> SEQHAQGADAVVDLNNELKTRREKLANLREQGIAFPNDFRRDHTSDQLHAEFDGKENEELEALNIEVAVAGRMMTRRIMGKASFVTLQDVGGRIQLYVARDDLPEGVYNEQFKKWDLGDILGAKGKLFKTKTGELSIHCTELRLLTKALRPLPDKFHGLQDQEARYRQRYLDLISNDESRNTFKVRSQILSGIRQFMVNRGFMEVETPMMQVIPGGAAARPFITHHNALDLDMYLRIAPELYLKRLVVGGFERVFEINRNFRNEGISVRHNPEFTMMELYMAYADYKDLIELTESLFRTLAQDILGKTEVTYGDVTLDFGKPFEKLTMREAIKKYRPETDMADLDNFDSAKAIAESIGIHVEKSWGLGRIVTEIFEEVAEAHLIQPTFITEYPAEVSPLARR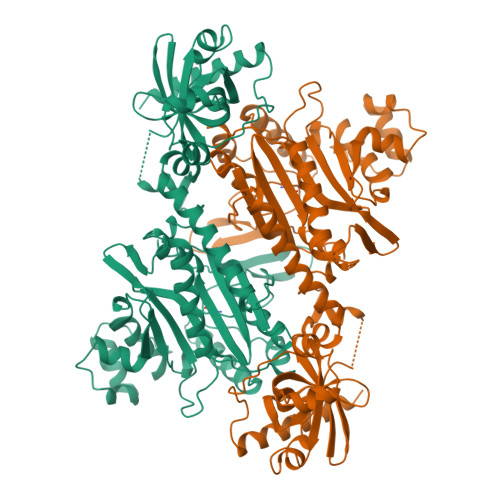NDVNPEITDRFEFFIGGREIGNGFSELNDAEDQAQRFLDQVAAKDAGDDEAMFYDEDYVTALEHGLPPTAGLGIGIDRMVMLFTNSHTIRDVILFPAMRPVK>[2x]MNGAIKVGAWGGNGGSAFDMGPAYRIISVKIFSGDVVDGVDVTFTYYGKTETRHYGGSGGTPHEIVLQEGEYLVGMAGEVANYHGAVVLGKLGFSTN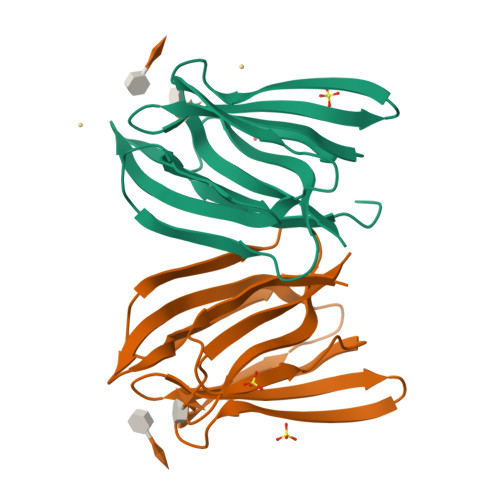KKAYGPFGNTGGTPFSLPIAAGKISGFFGRGGKFLDAIGVYLEP> ADTIVAVELDTYPNTDIGDPSYPHIGIDIKSVRSKKTAKWNMQDGKVGTAHIIYNSVDKRLSAVVSYPNADATSVSYDVDLNDVLPEWVRVGLSASTGLYKETNTILSWSFTSKLKSNSTHQTDALHFMFNQFSKDQKDLILQGDATTGTDGNLELTRVSSNGSPEGSSVGRALFYAPVHIWESSAATVSFEATFAFLIK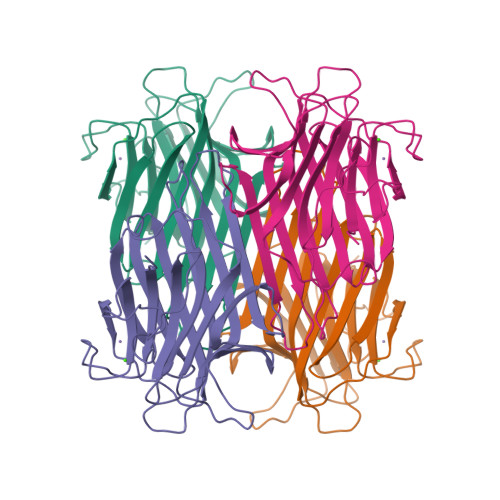SPDSHPADGIAFFISNIDSSIPSGSTGRLLGLFPDAN>GADLSEPFSLTEVQTAYMLGRNPQFELSGISPQTYFEYETELDIARLSRSFQKVIQRHPMLRAVILPEGKQQILRDVPEYEIEVESLVSMPPEKQAARLREERSRMIDHVFPLGQWPLFELKAFQLQEHTYLLCFRYDALLMDGASMNLVGQDLMHYYHQPDAQLPPLSFTFQDYMHIYDDMKRGTEYETAKAYWTNKLPDFPPAPSLLLAKDPAEIGTPNFQSLTTIITKDKWLKLRRLAQDKQVTPSALLCTVYGEVLAFWSNQRRLAINLTVFNRYPVHDEVEQIVGDFTSLILLDMDMDQKQPFFTKVEQTQSTLLDGLEHRHYDGVEFIRDYTRYHQMRPKAVMPIVFTSMLAGAGAFAWEEIGSLRHIHARTPQVYLDNVVIEKNGELLVSWNYVEELFDAEVMESMFTQFVELLDQLVEQGDINPLRISQKDY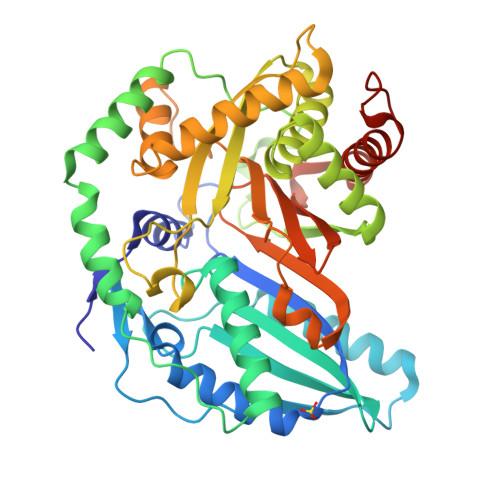ALIDQ[2x]(1S,2S,3Z,5S,8Z)-5-hydroxy-5,9-dimethyl-2-(propan-2-yl)cyclodeca-3,8-dien-1-yl 4-hydroxybenzoate | 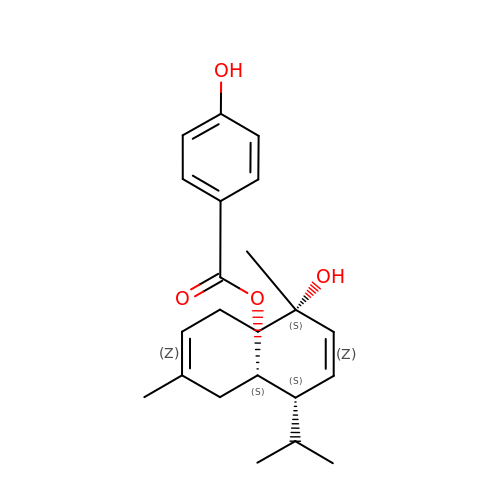C22 H30 O4 | AVRRAMZPNSQDIW-TUNDKXTFSA-N> MSKGTTSQDAPFGTLLGYAPGGVAIYSSDYSSLDPQEYEDDAVFRSYIDDEYMGHKWQCVEFARRFLFLNYGVVFTDVGMAWEIFSLRFLREVVNDNILPLQAFPNGSPRAPVAGAL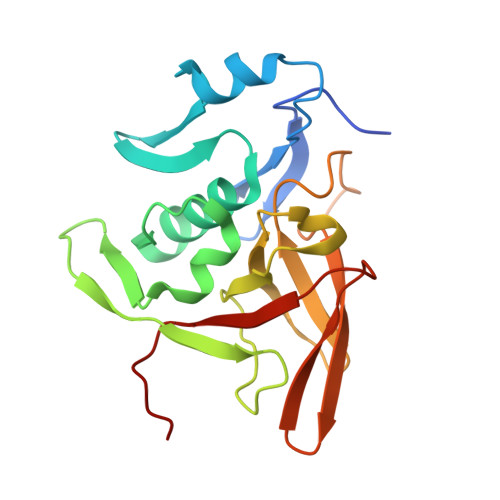LIWDKGGEFKDTGHVAIITQLHGNKVRIAEQNVIHSPLPQGQQWTRELEMVVENGCYTLKDTFDDTTILGWMIQTEDTEY>[4x]MGSSHHHHHHSSGGDESQARVLHMVGDKPVFSFQPRGHLEIGEKLDIIRQNLSPRRLSHVSGHRSYYLRGAGALLQHGLVNFT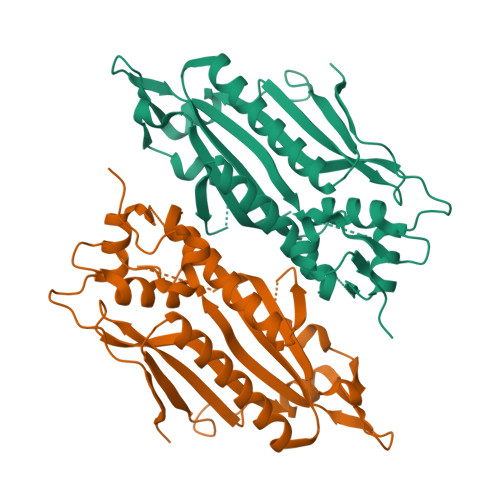FNKLLRRGFTPMTVPDLLRGAVFEGCGMTPNANPSQIYNIDPARFKDLNLAGTAEVGLAGYFMDHTVAFRDLPVRMVCSSTCYRAETNTGQEPRGLYRVHHFTKVEMFGVTGPGLEQSSQLLEEFLSLQMEILTELGLHFRVLDMPTQELGLPAYRKFDIEAWMPGRGRFGEVTSASNCTDFQSRRLHIMFQTEAGELQFAHTVNATACAVPRLLIALLESNQQKDGSVLVPPALQSYLGTDRITAPTHVPLQYIGPNQPRKPGLPGQPAVS>QEDEDGDYEELVLALRSEEDGLAEAPEHGTTATFHRCAKDPWRLPGTYVVVLKEETHLSQSERTARRLQAQAARRGYLTKILHVFHGLLPGFLVKMSGDLLELALKLPHVDYIEEDSSVFAQSIPWNLERITPPRYRADEYQPPDGGSLVEVYLLDTSIQSDHREIEGRVMVTDFENVPEEDGTRFHRQASKCDSHGTHLAGVVSGRDAGVAKGASMRSLRVLNCQGKGTVSGTLIGLEFIRKSQLVQPVGPLVVLLPLAGGYSRVLNAACQRLARAGVVLVTAAGNFRDDACLYSPASAPEVITVGATNAQDQPVTLGTLGTNFGRCVDLFAPGEDIIGASSDCSTCFVSQSGTSQAAAHVAGIAAMMLSAEPELTLAELRQRLIHFSAKDVINEAWFPEDQRVLTPNLVAALPPSTHGAGWQLFCRTVWSAHSGPTRMATAIARCAPDEELLSCSSFSRSGKRRGERMEAQGGKLVCRAHNAFGGEGVYAIARCCLLPQANCSVHTAPPAEASMGTRVHCHQQGHVLTGCSSHWEVEDLGTHKPPVLRPRGQPNQCVGHREASIHASCCHAPGLECK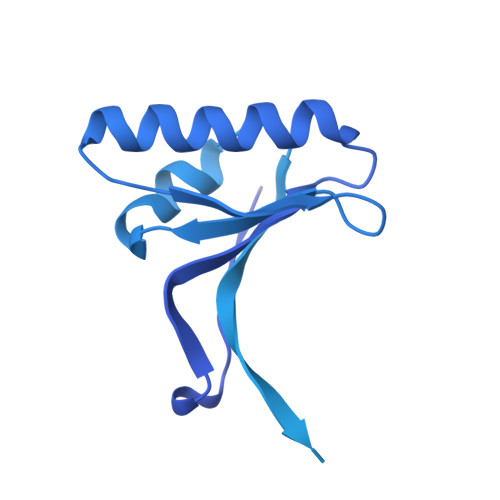VKEHGIPAPQEQVTVACEEGWTLTGCSALPGTSHVLGAYAVDNTCVVRSRDVSTTGSTSEEAVTAVAICCRSRHLAQASQELQKGNSADIQHSGGRSSLEGPRFEGKPIPNPLLGLDSTRTGHHHHHH[2x]> SSEELLKQALQQAQQLLQQAQELAKKGGGEELLKQALQQAQQLL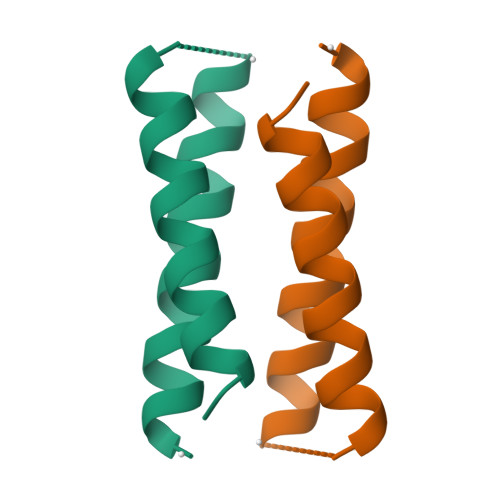QQAQELAKKGGGGEELLKQALQQAQQLLQQAQELAKKGGGEELLKQALQQAQQLLQQAQELAKK> MDEYVQELKGLIRKHIPERCEFGHQKVTFLSQVHPSPLLTEGFKLLSSLVELESCEAHACQANTDQRFVDVILSDNGILCPTLPKVIPDGFKLTGKTLILLETFVRVNPDEFEKKWKADMSKLLNLKHDLQKSGVTLVPIVDGRSNYNNRFVADWVIERIRWLLIEILKASKSMLEIDIEDQEYQRLIHSLSNVKNQSLGLENLEHLKRNSLDYDERLNESLFIGLKGDIRESTVREELIKLKLWFKDEVFSKGLGKFKLTDRRELLESLSSLGAHLDSDVSSCPFCNNKLMEIVYNVTFSCVERTDGVATVDQQFSTTHSNIEKHYLSVLSLCNKIKGLKVFNTRRNTLLFLDLIMVNLMVDISDSCQDAIESLRKSGLIVGQMVMLVNDRVLDILEAVKLIRKKIGTNPNWVKNCSKILERSHPEIWHHLSTLIKQPDFNSLISIAQHLVSDRPIMRYSVERGSDKICRHKLFQEMSSFEQMRLFKTLSSISLSLINSMKTSFSSRLLVNEREFSKYFGNVRLRECYAQRFYLAESLVGFLFYQKTGERSRCYSVYLSDNGVMSEQGSFYCDPKRFFLPVFSDEVLAGMCEEMTSWLDFDTGLMNDTGPILRLLVLAILCSPSKRNQTFLQGLRYFLMAFANQIHHIDLTSKLVVECKSSSEVVVQRLAVGLFIRLLSGESDASLFFSRRFKYLLNVSYLCHLITKETPDRLTDQIKCFEKFIEPKVKFGCAVVNPSLNGKLTVDQEDIMINGLKKFFSKSLRDTEDVQTPGVCKELLNYCVSLFNRGKLKVSGELKNNPFRPNITSTALDLSSNKSVVIPKLDELGNILSTYDKEKLVSACVSSMAERFKTKGRYNLDPDSTDYLILKNLTGLVSAGPKAKSTQEELSLMYEALTEEQVESFNEIKHDVQVALAKMADNSVNTRTKNLGRADNSVKNGNNPLDNLWSPFGVMKEIRAEVSLHEVKDFDPDVLPPEVYKELCDAVYKSSEKCNFFLEGVLDVCPLGLLLKNLTTSSYVDEEYFMCFKYLLIQGHFDQKLGSYEHKSRSRLGFTDETLRLKDEVRLSIRESNSEAIADKLDKSYFTNAALRNLCFYSEDSPTEFTSISSNSGNLKFGLSYKEQVGSNRELYVGDLNTKLMTRLVEDFSEAVGNSMKYTCLNSEKEFERAICDMKMAVNNGDLSCSYDHSKWGPTMSPALFLALLQMLELRTPVDRSKIDLDSVKSILKWHLHKVVEVPINVAEAYCIGKLKRSLGLMGCGSTSLSEEFFHQTMQLNGQIPSHIMSVLDMGQGILHNTSDLYGLITEQFLCYALDLLYDVIPVSYTSSDDQITLIKTPSLDIEGGSDAAEWLEMICFHEFLSSKLNKFVSPKSVIGTFVAEFKSRFFVMGEETPLLTKFVAAALHNVKCKTPTQLSETIDTICDQCIANGVSTKIVTRISKRVNQLIRYSGYGETPFGAIEDQDVKDWVDGSRGYRLQRKIEAIFHDDKETSFIRNCARKVFNDIKRGRIFEENLINLIGRGGDEALTGFLQYAGCSEQEVNRVLNYRWVNLSSFGDLRLVLRTKLMTSRRVLEREEVPTLIKTLQSKLSRNFTKGVKKILAESINKSAFQSSVASGFIGFCKSMGSKCVRDGKGGFLYIKEVYSGVSACTCEICALKPKIIYCNNSLNKVSQFSKPILWDYFSLVLTNACELGEWVFSTVKEPQKPLVLNNQNFFWAVKPKVVRQIEDQLGMNHVLQSIRRNYPVLFDEHLTPFMNDLQVSRTMDSGRLKFLDVCIALDMMNENLGIISHLLKTRDNSVYIVKQSDCALAHIRQSSYTDWELGLSPQQICTNFKTQLVLSSMVNPLVLSTSCLKSFFWFNEVLELEDDSQIELAELTDFALMVKNQNVSRAMFVEDIAMGYVVSNFEGVRISLSNVMVDGVQLPPQEKAPDIGELFGLKAENVIVGLVVQIDHVRMSTKFKLKRKMVYSFSLECIMDVGEIQNKEVILKVVAVDQSVSGSGGNHMLLDGVSVVASLPLFTGQASFDLAAMLIESNLAGSNDNFLMRNVTLDLGGFSPELSDKYSYRLSGPENQEDPLVLKDGAFYVGGERLSTYKVEFTGDLVVKALGALEDDESVVSMLHQLWPYLKATSQVILFQQEDFTIVHDLYKKQLTKSIESFGEWIEFTNFKVAYSKSLKELVISDTQGSFRLKGVMCRPLASTPQVEDIE;> MGNCNKPPKRPPNTQTSSNQPSAEFRRTAPPSLYGRYNCKCCWFADTNLITCNDHYLCLRC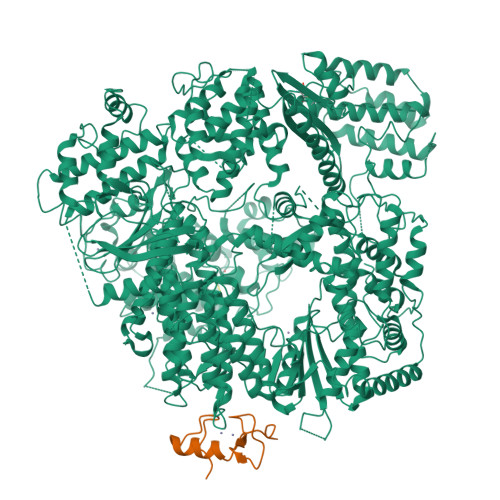HQTMLRNSELCHICWKPLPTSITVPVEPSAPPP TOSYL-D-PROLINE | C12 H15 N O4 S | 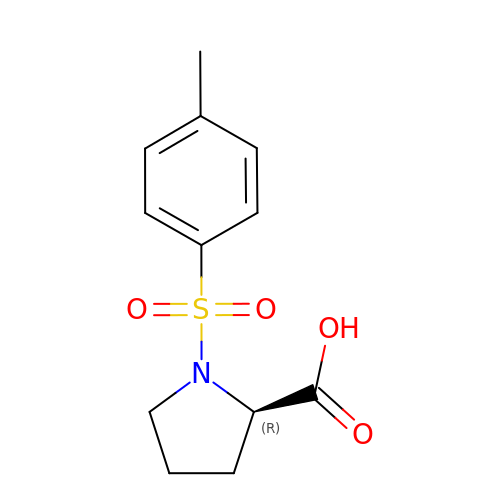CGPHGPCHVUSFFA-LLVKDONJSA-N> MIEIKDKQLTGLRFIDLFAGLGGFRLALESCGAECVYSNEWDKYAQEVYEMNFGEKPEGDITQVNEKTIPDHDILCAGFPCQAFSISGKQKGFEDSRGTLFFDIARIVREKKPKVVFMENVKNFASHDNGNTLEVVKNTMNELDYSFHAKVLNALDYGIPQKRERIYMICFRNDLNIQNFQFPKPFELNTFVKDLLLPDSEVEHLVIDRKDLVMTNQEIEQTTPKTVRLGIVGKGGQGERIYSTRGIAITLS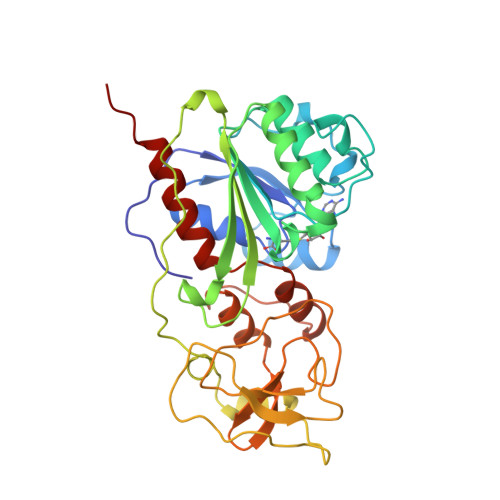AYGGGIFAKTGGYLVNGKTRKLHPRECARVMGYPDSYKVHPSTSQAYKQFGNSVVINVLQYIAYNIGSSLNFKPY> KGPAEDTYSTSWTNVNYASDSLESHNLDIYLPKEQKTAYKAIIIIYGSAWFANNAKAMASASIGAPLLKAGFAVISINHRSSMEAIWPAQIQDVKAAIRYVRSNAAKYNIDPSFIGITGFSSGGHLSAFAGVTNGVKTLTSGDLTVDIEGSLGNYLSTGSHVDAVVDWFGPVDMAHMSNCVAPNDASTPEAVLIGKKDPREEPDWVKLISPINFVDKDDPDILIIHGDADNVVPHCQSVNLKNVYDNAGAKATFISVPGGGHGPGCFDTQYFKD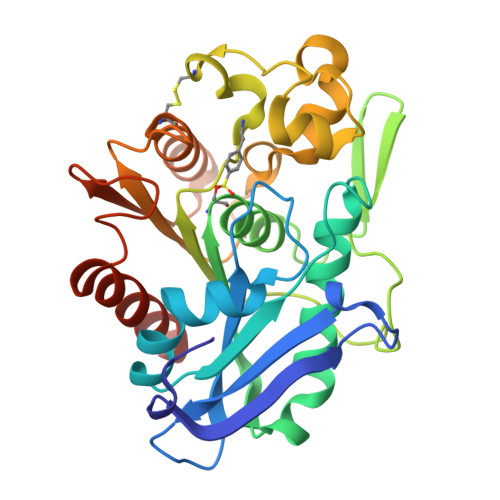MTDFFTEQSTKLEHHHHHH>EVVRPEVNRTGTVDICQGPMELIFSVSRTSSGATGERISLKNTLSIVSMENGGKPGTYEWSFPANESWPEIQFLLQNREFVSKYYADVVQTPGELVVEYRCPVPQFNCTITHRWKGETIMSFDGAIQTIRSVTSEYTTKNEDTLVKYIRGLNVTLLTDNAKSIEHRWTEICKKLKDADRPDDNQYTLEDDILEDDIEMDIVQCQMTTQVPLKYHMTVWSAGRDSRAIALSADYYTDIEVASYLPVNRSQILNTTCEITSSSGWTVRLRFSEEMVAASKARQAQKRPLLPVEPHGFMSDEHGPAFVQRTINDSRLTLVPR[2x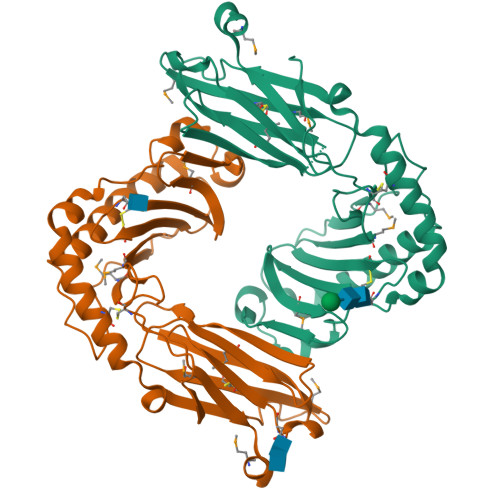]>TSLREEEESQDNPFYFNSDNSWNTLFKNQYGHIRVLQRFDQQSKRLQNLEDYRLVEFRSKPETLLLPQQADAELLLVVRSGSAILVLVKPDDRREYFFLTSDNPIFSDHQKIPAGTIFYLVNPDPKEDLRIIQLAMPVNNPQIHEFFLSSTEAQQSYLQEFSKHILEASFNSKFEEINRVLFEEEGQQEGVIVNIDSEQIKELSKHAKSSSRKSLSKQDNTIGNEFGNLTERTDNSLNVLISSIEMEEGALFVPHYYSKAIVILVVNEGEAHVELVGPKGN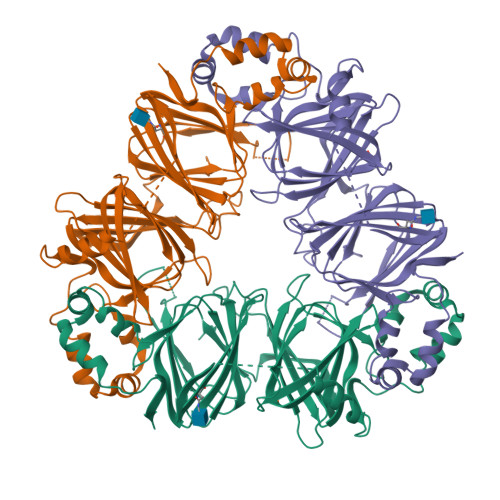KETLEYESYRAELSKDDVFVIPAAYPVAIKATSNVNFTGFGINANNNNRNLLAGKTDNVISSIGRALDGKDVLGLTFSGSGDEVMKLINKQSGSYFVDAHHHQQEQQKGRKGAFVY[3x]> MGCQSTQLQTPAPDTGGIVELNRQLGRGVNLGNALEAPWEGAWGVRLEEGFFELIREAGFKTIRLPVSWTHHAGRAAPYTIDPAFFSRVDWAVTQATRRGLNIVVNVHHYDELNANPQAEEARYLSIWRQIAERYRNQPGSVYFELLNEPHGRFNDNPQLWNDLLAKALRVVRESNPSRAVIVGPVGWNSLWRLSELRLPDDPNLIVTFHYYDPLEFTHQGAEWLNPVPPTGVVWHQQNAIAQAMEFAQRWAEQNRRPIFVGEFGAYEKGDLDSRVRWTGAVRSELEKRNFSWAYWEFAAGFGIYDRTTRQWRTPLLKALVPEQPKLKLAAALEHHHHHH

Here, by solving the crystal structure, it is shown that MtGlu5 from Meiothermus taiwanensis WR-220, a GH5-family endo-β-1,4-glucanase (EC 3.2.1.4), has a bipartite architecture consisting of a Cel5A-like catalytic domain with a (β/α)8 TIM-barrel fold and an inserted CBM29-like noncatalytic domain with a β-jelly-roll fold. MtGlu5 contains a Cel5A-like CD similar to TmCel5A from Thermotoga maritima, but has an additional novel domain inserted into an internal site in the CD. Unlike other known cellulases with CBMs at the termini, this inserted CBM in the newly identified MtGlu5 acts in synergy with the CD, as demonstrated by ITC experiments.

To investigate the origin of the disparity in catalytic efficiency between ΔCBM and MtGlu5, we crystallized ΔCBM and solved the structure by molecular replacement using the CD of MtGlu5 as a search model. The orthorhombic P212121 crystal contained one molecule of ΔCBM in its asymmetric unit. The apo-form structure of ΔCBM displayed an intact TIM-barrel fold. The crystal structure of ΔCBM presents almost the same polypeptide conformation as observed in the CD of MtGlu5, with an r.m.s.d. of 0.28 Å for 260 pairs of Cα atoms. In MtGlu5 (and also in TmCel5A) the β6–α6 loop is 30 residues long and contains the substrate-binding Trp224 (Trp210). Direct elimination of the CBM from MtGlu5 resulted in a shorter connection between this loop and the α6 helix, the equivalent of which in TmCel5A has one additional turn. Although the overall fold remained intact, the lack of flexibility in the tightened-up loop would probably have reduced the catalytic efficiency of ΔCBM. Similar results were obtained using the soluble substrate CMC. The kinetic data indicated that without the CBM domain, the K m of ΔCBM increased nearly ninefold and the k cat decreased by more than tenfold. The lower enzymatic activity of ΔCBM is not due to structural damage to the catalytic center, the integrity of which was demonstrated by analyzing the hydrolyzed products using mass spectroscopy.> ANI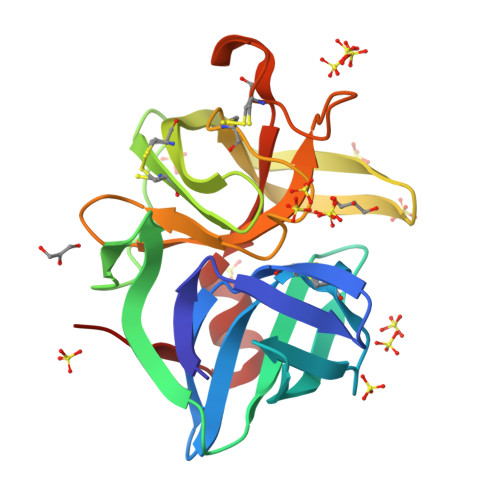VGGIEYSINNASLCSVGFSVTRGATKGFVTAGHCGTVNATARIGGAVVGTFAARVFPGNDRAWVSLTSAQTLLPRVANGSSFVTVRGSTEAAVGAAVCRSGRTTGYQCGTITAKNVTANYAEGAVRGLTQGNACMGRGDSGGSWITSAGQAQGVMSGGNVQSNGNNCGIPASQRSSLFERLQPILSQYGLSLVTG> SGRSRLLEDFRNQRYPNLQLRDLANHIVEFSQDQHGSRFIQQKLERATAAEKQMVFSEILAAAYSLMTDVFGNYVIQKFFEFGTPEQKNTLGMQVKGHVLQLALQMYGCRVIQKALESISPEQQQEIVHELDGHVLKCVKDQNGNHVVQKCIECVDPVALQFIINAFKGQVYSLSTHPYGCRVIQRILEHCTAEQTTPILDELHEHTEQLIQDQYGNYVIQHVLEHGKQEDKSILINSVRGKVLVLSQHKFASNVVEKCVTHATRGERTGLI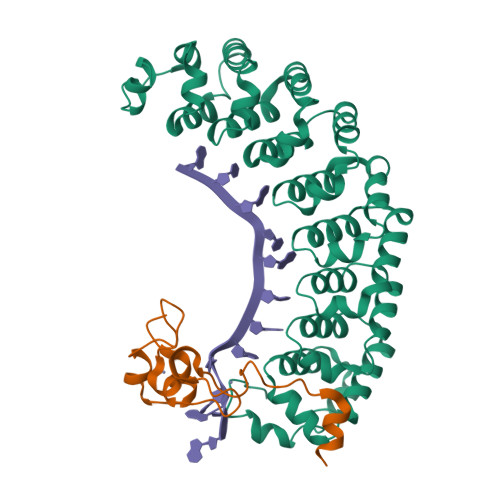DEVCTFNDNALHVMMKDQYANYVVQKMIDVSEPTQLKKLMTKIRPHMAALRKYTYGKHINAKLEK;> SRGASNSSNNNNNNNKVYKRYNSKAKEISRHCVFCENNNEPEAVINSHSVRDNFNRVLCPKLRTYVCPICGASGDSAHTIKYCPKKPIITMEDAIKAESFRLAKSSYYKQQMKV> ASTFSGVQSLPKFEIHDVRDDPAEGTMTRVAVDGKLLLISQYPQLGP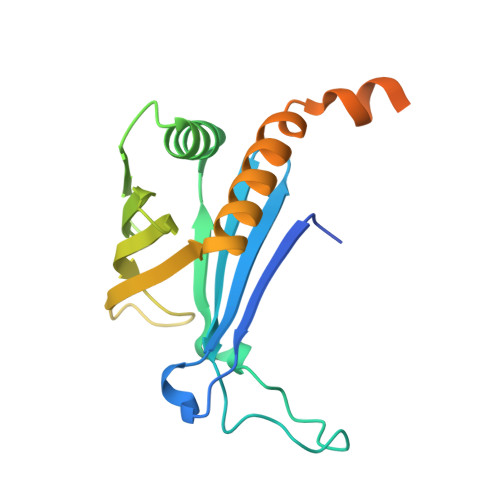RKVDPNDLSPQFDADRRISVRLRHVDLAYLVGVCKERVPRHRMETKAYTLDFEKSAQGYHLHGKVHRVASQRMEDWSVKFDNHFAVTLEHFLESALDESFGFRQHYATRAAEGGEKIAATSSAEGGARRKRSVSDTSRYH>MISDPQVLGFIARTEAAYPPEANGASAADNRRFYDAMCAVFRGPRPPGLVVGDRRIGGVPCRVYGADSAVSVVYVHGGGFVVGGLDSHDDVCAEIADATGLQVIAIDYRLAPEHRWPAQIQDVQAVWDALDRPAVIAGDSAGGMLSAALCLSRRGQRQPLGQVLIYPGLGGDGSAPSYRENAGAPLLRTEDLATYHAALHGDGPVDPLALPLQVEDLAGVAPAFVVSADVDPLRDDARDYVQRLRAAGVAAEWRNE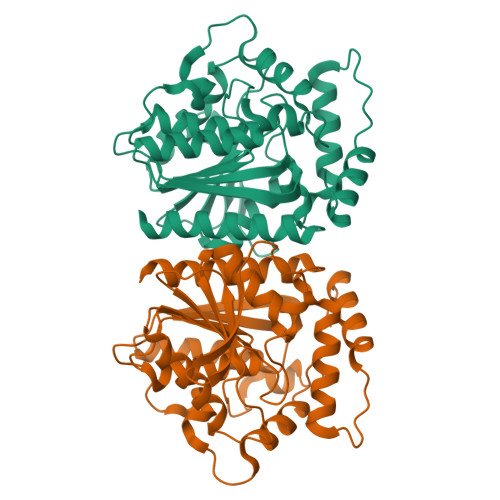PELPHGYLRARRESDRARRSFQAILSAIMRFAVRG[2x]> ETSQCKILRCNAEYVSSTLSLRGGGSSGALRG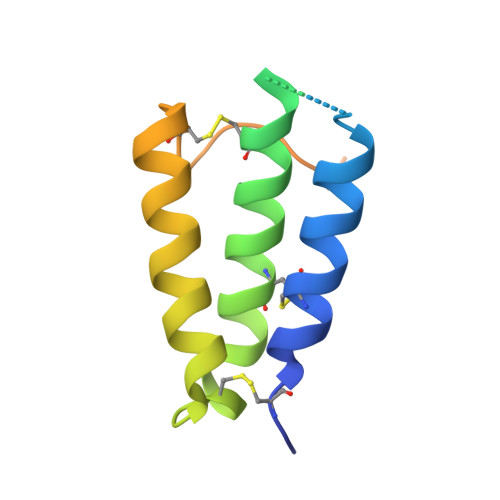GGGGGRGGGVGSGGLCRALRSYALCTRRTARTCRGDLAFHSAVHGIEDLMIQHNCSRQGPTAPPPPRGPALPGAGSGLPAPGTKHHHHHH> MGAQVSTQKSGSHETGNVATGGSTINFTNINYYKDSYAASA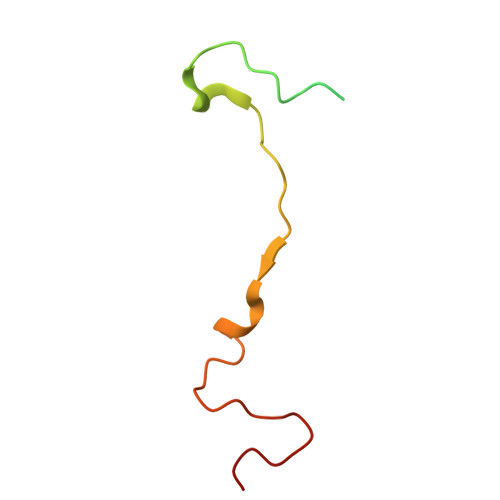TRQDFTQDPKKFTQPVLDSIRELSAPLN> GMTSDNAAFEGTF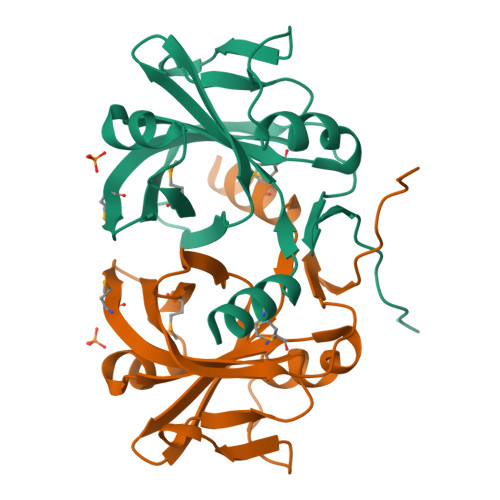KEMFRRHAAGVAIITVNYNGTPYGFTATSVASLSAQPPRFTFNMARSSSSWPAIANTTHIGVHMLGLDNQELADRFARTKNRFEGDHWELGPYEVPILKDVAGWLIGKIQMRLSFENNAVVVVEVVEGQVGEDGTPLLYHSGAYSQPVPLDYEI(Z)-4-(1-{4-[2-(DIMETHYLAMINO)ETHOXY]PHENYL}-5-HYDROXY-2-PHENYLPENT-1-ENYL)PHENOL 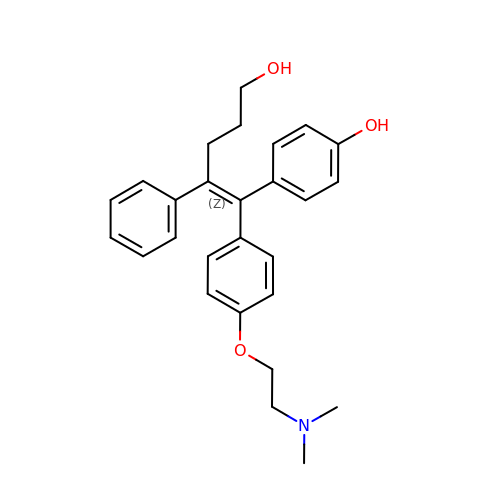| C27 H31 N O3 | ZVSFNBNLNLXEFQ-RQZHXJHFSA-N> MSKKLLSVLFGASLAALALSPTAFAADQGGSDGKDGEDGKPGPVGLDISQATTLKATLEDVKIDNGTVSVDIVLTNANGVPVTG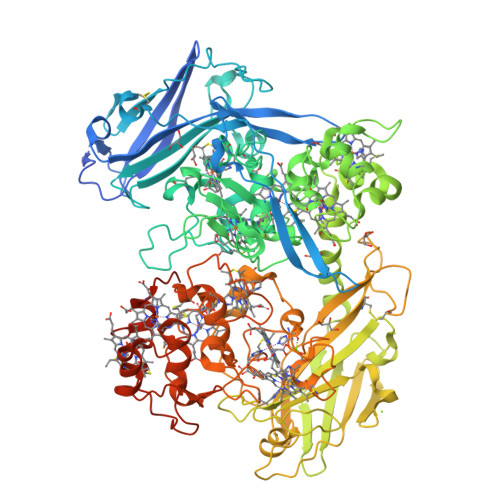LEQYAQINAIGLGIAKLTPESGKGYKTPQWVSYINSVKAADPARSLANYSYTDGKDSAGNPITKEVKFTPGDAIQANIESSCKTTCLTVVDSGVYRYTFQTNLSTLPAIEGLDLTYDPTLIHRITLELQTDGSKDAKLVNSHIDFLPSDNFRVAKETETRTVVDLEANCIKCHSTNYSDTSSTAKPLALHGGRRIGIANCQVCHTSYSKDPETGSPLDMGAMVHAIHKGTYAMVGYSGTAYDFSGTMAKAAAESGYPQYREGKDVSERVTLPVSIGNCQSCHSTDDKGPVDAASFKHHKGLACASCHMSGFNPVDNSEWLTPPEGQKDRGFVGNYFHYYATPEIDGIPGVNLVHVFQNGGCASCHAEQGEEGSAKYHLAKANATKLLRTEYAYKLENGTFDVAKGELTFTVNWHSDVAPHQDPKVKEFWVSLTAFNGTEYTMGPRPSNGTLGRSENRISVNLAKVETNANLTAVPNGSKVTYTLTGIKAVIGTSSVPYKQIVSIGKGFMDGKLLICANSAELDPTMDAAIDCSNTEAPIYEVIVGSNKASFSADASNVTARSIVISEAKCANCHGEKADFSASHALTHAADKPDNSCGTCHSAVPNTAVALADGSCVACHNGAPAHSKKPFERGFDFKVMIHQIHADTRSVRRLTTDAATFPENPANCAACHDKGQLSLATLGNKPAFLASTGEYSPTVAACASCHATTATDSAVIGHFETNGGVYNAAAGTYTPGSETCATCHGEGKSFGVDKVHPVKYKGELKLEGKPIPNPLLGLDSTRTGHHHHHH> MAMKREQTIENLYQLAQLTQQVQADRIEIVLEERRDEHFPPMSKALMETRSGLTRRKLDEAIAKMEEAGHQFTKNNANHYSISLSEAHMLMDAAGVPKFHERKKNNENKPWIINVQNQKGGTGKSMTAVHLAACLALNLDKRYRICLIDLDPQGSLRLFLNPQISLAEHTNIYSAVDIMLDNVPDGVQVDTEFLRKNVMLPTQYPNLKTISAFPEDAMFNAEAWQYLSQNQSLDIVRLLKEKLIDKIASDFDIIMIDTGPHVDPLVWNAMYASNALLIPCAAKRLDWASTVNFFQHLPTVYEMFPEDWKGLEFVRLMPTMFEDDNKKQVSVLTEMNYLLGDQVMMATIPRSRAFETCADTYSTVFDLTVNDFEGGKKTLATAQDAVQKSALELERVLHSHWSSLN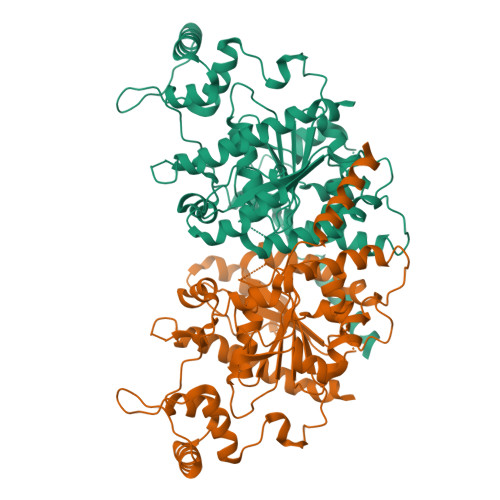QG>[2x]MADETIAIVDADATAETRSLLSYLDGVRGEGILFGHQHTTSFGLTTGPTDGTTSDVKNVTGDFPAVFGWDTLIIEGNERP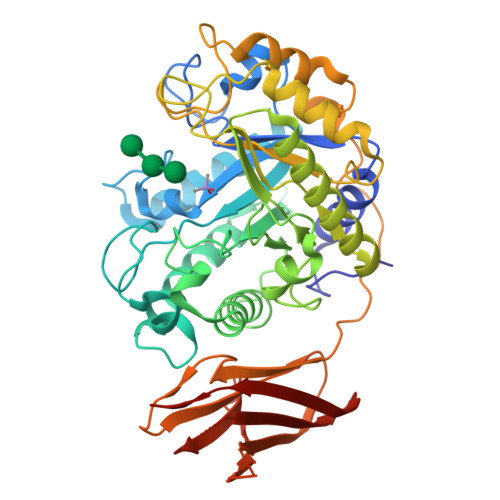GLAENTRDENIALFADYIRKADAIGGVNTVSAHVENFVTGGSFYDTSGDTLRAVLPGGSHHAELVAYLDDIAELADASRRDDGTLIPIVFRPWHENAGSWFWWGAAYGSPGEYQELYRFTVEYLRDVKGVSNFLYAWGPGGGFGGNRDVYLRTYPGDAFVDVLGLDTYDSTGSDAFLAGLVADLRMIAEIADEKGKVSAFTEFGVSGGVGTNGSSPAQWFTKVLAAIKADPVASRNAYMETWANFDAGQHFVPVPGDALLEDFQAYAADPFTLFASEVTGAFDRTVAAAPAQPVVHIASPADGARVASAPTTVRVRVGGTDVQSVTVEVAQGGTVVDTLDLAYDGALWWTAPWSPTSAQLDNSTYTVTATATTAAGTLDVTNEVAAALEHHHHHH> SVSAGEKPPRLYDRRSIFDAVAQSNCQELESLLPFLQRSKKRLTDSEFKDPETGKTCLLKAMLNLHNGQNDTIAL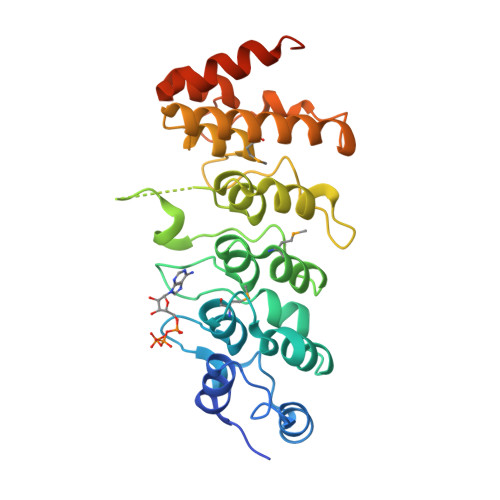LLDVARKTDSLKQFVNASYTDSYYKGQTALHIAIERRNMTLVTLLVENGADVQAAANGDFFKKTKGRPGFYFGELPLSLAACTNQLAIVKFLLQNSWQPADISARDSVGNTVLHALVEVADNTVDNTKFVTSMYNEILILGAKLHPTLKLEEITNRKGLTPLALAASSGKIGVLAYILQREIHEPECRHAAAHHHHHH N-[1-(2-Chloroacetyl)piperidin-4-yl]-5-cyclopropyl-1,2-oxazole-3-carboxamide | 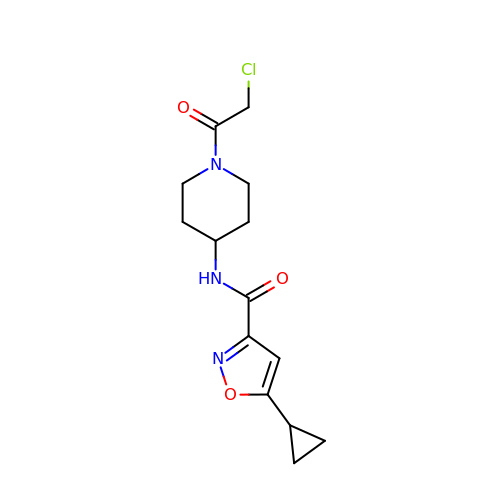C14 H18 Cl N3 O3 | OENTXAYVUCLRJQ-UHFFFAOYSA-N>[2x]DKWEMERTDITMKHKLGGGQYGEVYVGVWKKYSLTVAVKTLKEDTMEVEEFLKEAAVMKEIKHPNLVQLLGVCTLEPPFYIVTEYMPYGNLLDYLRECSREEVTAVVLLYMATQISSAMEYLEKKNFIHRDLAARNCLVGENHVVKVADFGLSRLMTGDTYTAHAGAKFPIKWT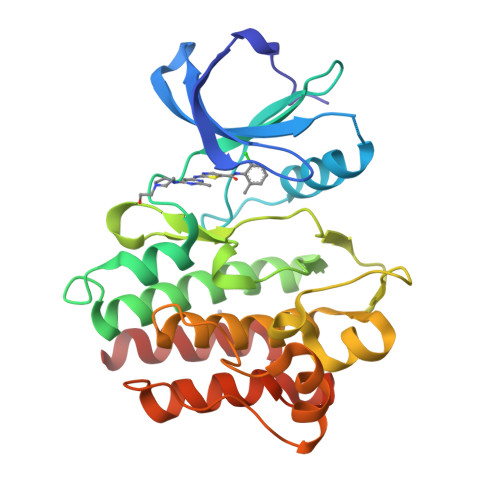APESLAYNTFSIKSDVWAFGVLLWEIATYGMSPYPGIDLSQVYDLLEKGYRMEQPEGCPPKVYELMRACWKWSPADRPSFAETHQAFETMFHDS>[4x]MTAVEFIEPLTHEEGVSQATKLFVDTYGAAPEGVWAAPGRVNLIGEHTDYNAGLCLP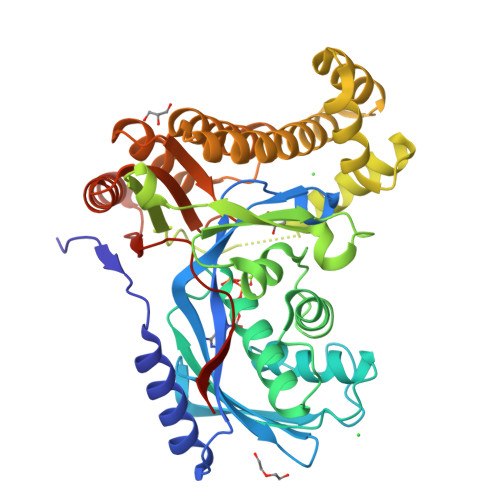IALPHRTFIALKPREDTKVRVVSGVAPDKVAEADLDGLKARGVDGWSAYPTGVAWALRQAGFDKVKGFDAAFVSCVPLGSGLSSSAAMTCSTALALDDVYGLGYGDSDAGRVTLINAAIKSENEMAGASTGGLDQNASMRCTEGHALLLDCRPELTPLENVSQQEFDLDKYNLELLVVDTQAPHQLNDGQYAQRRATCEEAAKILGVANLRVTADGISKADDQFQALKETLDALPDETMKKRVRHVVTEIERVRSFVRAFAQGDIKAAGRLFNASHDSLAADYEVTVPELDIAVDVARKNGAYGARMTGGGFGGSIIALVDKGQGHEIAQKIADRFEKEGFNAPRALPAFAAASASREAKLAAALEHHHHHH>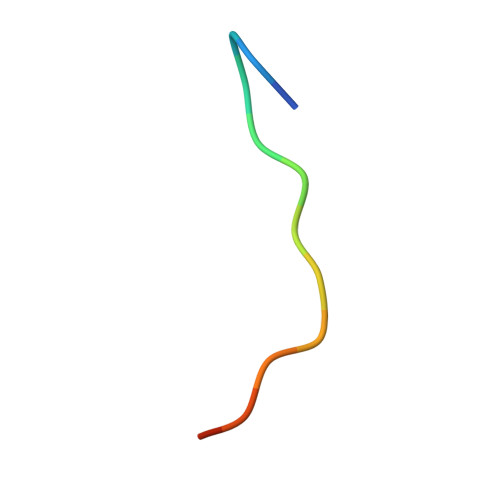 YPGGSTPVSSANMM> AKLDKEQVIDNALILLNEVGIEGLTTRKLAQKIGVEQPTLYWHVKNKRALLDALAETILQKHHHHVLPLPNETWQDFLRNNAKSFRQALLMYRDGGKIHAGTRPSESQFETSEQQLQFLCDAGFS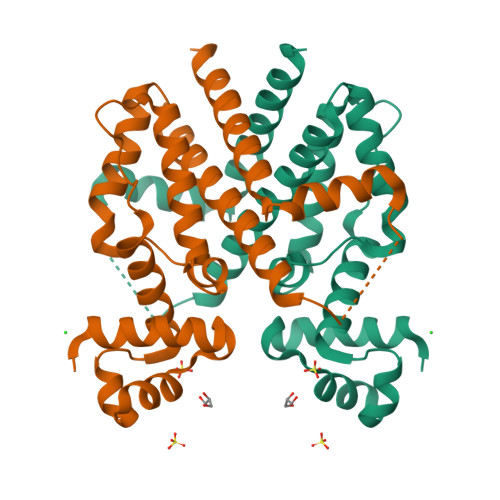LSQAVYALSSIAHFTLGSVLETQEHQESQKEREKVETDTVAYPPLLTQAVAIMDSDNGDAAFLFVLDVMISGLETVLKSAK>SNAPDAGPSTGPSGSPDMQPMATTAPLPEAPATCDLAALPARDKLAQLLTVGVTDAADARAVVADHHVGGIMIGSWTDLSMLTDGSLGDIAASAAPLPLAVSVDEEGGRVSRLASLIGSQPSARELARTKTADEVYGIALDRGRKMRDLGVTVDFAPVVDVTDAAADTVIGDRSFGSDPAVVTEYAGAYARGLRDAGVLPVLKHFPGHGHASGDSHTGGVTTPPLDVLMGDDLVPYRTLTGQAPVAVMVGHMQVPGLTGSDPASLSPAVYNLLRSGGYGGPGFGGLVYTDDLSSMGAINQRYGVADAVLRALQAGADNALWITTAEVPAVLDRLEQALASG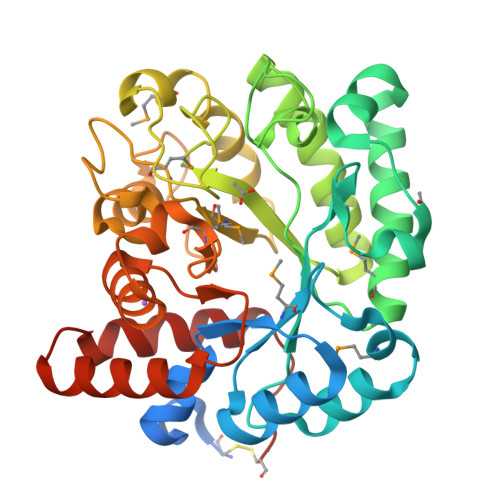ELNQGAVDASLQRNAAVKGPLRCG[3x]> MVSVINTVDTSHEDMIHDAQMDYYGTRLATCSSDRSVKIFDVRNGGQILIADLRGHEGPVWQVAWAHPMYGNILASCSYDRKVIIWREENGTWEKSHEHAGHDSSVNSVCWAPHDYGLILACGSSDGAISLLTYTGEGQWEVKKINNAHTIGCNAVSWAPAVVPGSLIDHPSGQKPNYIKRFASGGCDNLIKLWKEEEDGQWKEEQKLEAHSDWVRDVAWAPSIGLPTSTIASCSQDGRVFIWTCDD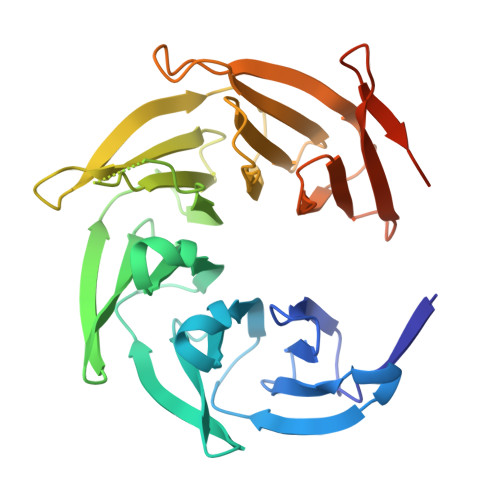ASSNTWSPKLLHKFNDVVWHVSWSITANILAVSGGDNKVTLWKESVDGQWVCISDVNKGQGSVSASVTEGQQNEQ>[2x]SMKGSGQIQLWQFLLELLADRANAGCIAWEGGHGEFKLTDPDEVARRWGERKSKPNMNYDKLSRALRYYYDKNIMSKVHGKRYAYRFDFQGLAQACQPPPAH

The Ets transcription factor family consists of 28 genes in humans containing the evolutionarily conserved 85 amino acid Ets DNA-binding domain, originally identified as a viral oncogene (E26 transformation-specific). The Ets domain is a variant helix-turn-helix (winged helix) structure, comprising three α-helices and a four-stranded antiparallel β-sheet. Here, we present the crystal structures of the Ets domains of the entire PEA3 subfamily (Etv1, Etv4, and Etv5) together with the structure of the Erg family member (Fev). Furthermore, a new Ets dimerization interface linked by a redox-sensitive disulfide bond is identified, and this dimerization is shown to result in a significant inhibition of DNA binding, potentially linking Ets transcription factors with cellular redox regulatory mechanisms.

Fev lacks additional domains and has a restricted tissue expression. Crystals were obtained from constructs that contained the Ets domain, Etv1 (encompassing amino acids 326–429), Etv4 (encompassing amino acids 338–470), and Fev (encompassing amino acids 42–141). Etv1, Etv4, and Fev display the typical fold of the Ets domain, which contains three α-helices (α1–3) flanking a four-stranded β-sheet, with an additional C-terminal helix (α4). The structures are highly similar (typical root mean square deviation of 1.0 Å over ∼90 residues), with the main difference being a two-amino acid deletion in Fev, linked to a shift of 30° in the orientation of the C-terminal α4 helix in the Fev structure compared with the other structures. Similar transitions occur in the Fev structure where Asp-99, Arg-103 and Tyr-107 adopt different rotamers, and the disordered Arg-106 and Lys-111 become ordered upon DNA binding. Similarly, an analysis of the crystal contacts in both the Fev and Fev-DNA crystals reveals an interface that includes the same components (α1 and α4 and the β1-β2 loop) as that of the other three Etv proteins. However, the dimer interfaces in Etv1/4/5 and in Fev are not equivalent; rather, they differ by a relative rotation of ∼90°, reflecting the different orientations of the α4 helix. The contact area for the Fev dimerization interface is ∼700 Å2, spans 21 residues, and accounts for 12.5% of the monomer accessible surface area. Similar to Etv1, the interface is dominated by contacts from hydrophobic residues, a single hydrogen bond (Asp-59–His-72), and an intermolecular disulfide bond between Cys-135 and its symmetry mate. We have been unable to test whether Fev also forms disulfide-linked homodimers, as our Fev constructs did not produce soluble protein in the Rosetta-gamiTM 2 E. coli cells.> TPVSEKQLAEVVANTITPLMKAQSVPGMAVAVIYQGKPHYYTFGKADIAANKPVTPQTLFELGGISKTFTGVLGGDAIARGEISLDDAVTRYWPQLTGKQWQGIRMLDLATYTAGGLPLQVPDEVTDNASLLRFYQNWQPQWKPGTTRLYANASIGLFGALAVKPSGMPYEQAMTTRVLKPLKLDHTWINVPKAEEAHYAWGYRDGKAVRVSPGMLDAQAYGVKTNVQDMANWVMANMAPENVADASLKQGIALAQSRYWRIGSMYQGLGWEMLNWPVEANTVVEGSDSKVALAPLPVAEVNPPAPPVKASWVHKTGSTGGFGSYVAFIPEKQIGIVMLANTSY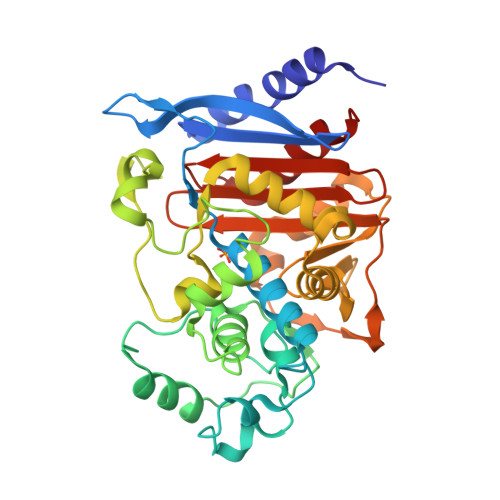PNPARVEAAYHILEALQ> HMLWARLVGLARLEA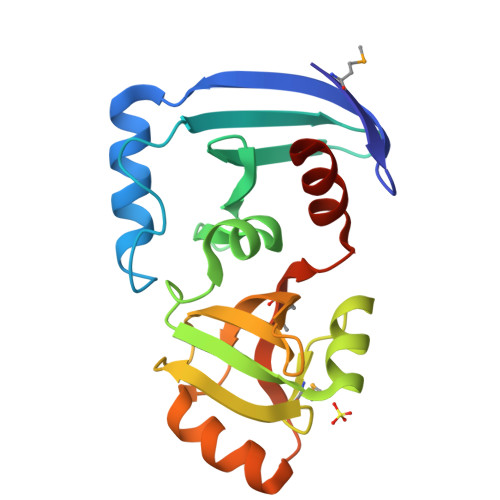RALSKKERRSLLERLKPYYTRIPFSEKADLRLVKARTDSGEYEIITVDGVPCLFEWSDGRIYPTLQCLKAFGVDWLKGVVLVDKGAAIALAKGAHLMIPGVVGVEGSFTRGDVVAALYHETRTPVMVGVAEVDSSALEKLYREKARGRAVRRVHRLGDALWELAQEVGKRLS> MGAMGKSKAEYYNAWSEWERNAPGGN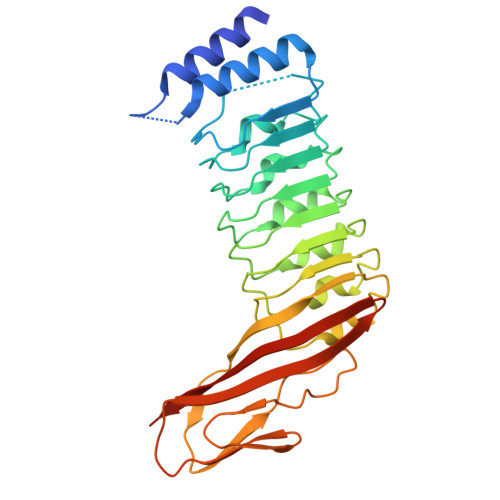GEQRGMAVSRLRDALDRQSHELELNNLGLSSLPGIQYLPNVTKLFLNGNKLTDIKPLANLKNLGWLFLDENKVKDLSSLKDLKKLKSLSLEHNGISDINGLVHLPQLESLYLGNNKITDITVLSRLTKLDTLSLEDNQISDIVPLAGLTKLQNLYLSKNHISDLRALAGLKNLDVLELFSQEILNKPINHQSNLVVPNTVKDTDGSLTTPAIISDDGDYEKPNVKWHLPEFTNEVSFIFRQLVNIGGSWAIFSGRVTQPLKEGSENLYFQ>MTVPTPY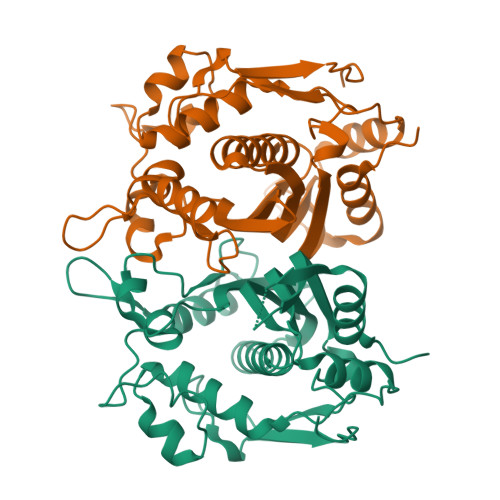EDLLRKIAEEGSHKDDRTGTGTTSLFGQQIRFDLNEGFPLLTTKKVHFHSVVGELLWFLQGDSNVKWLQDNNIRIWNEWADEDGELGPVYGVQWRSWPTPDGRHIDQISGALETLRNNPDSRRNIVSAWNVSELENMALPPCHLLFQLYVADGKLSCQLYQRSADMFLGVPFNIASYALLTHMFAQQAGLEVGEFIWTGGDCHIYDNHKEQVAEQLSREARPYPTLELNKAASMFEYSFDDITVSGYDPHPLIRGKVAV[2x]By contrast, in vertebrates the clustered protocadherins (Pcdhs) provide analogous cell-surface diversity, but in this case generated through stochastic alternative promoter choice. Biophysical measurements with domain-deleted proteins showed that Pcdhs also interact in cis, through a membrane-proximal dimer interface involving extracellular cadherin domain 6 (EC6) and potentially EC5. The specificity-determining cell-cell recognition interface of Pcdhs involves domains EC1–4, as shown experimentally through mutagenesis analysis and suggested by mutation correlation analysis.

The γA1EC1–4 crystal structure contained four molecules in the asymmetric unit: Two of which are arranged in an EC1–4-mediated antiparallel dimer, with all four EC domains involved in the dimer interaction (chains A and B); and two are arranged in an EC2–3-mediated antiparallel dimer, in which EC1 and EC4 are not involved in the dimer interaction (chains C and D). The EC2–3 portion of the dimer interaction is very similar between the two dimers in the structure (RMSD = 0.98 Å over 415 Cα’s) and closely resembles the partial interaction observed in the previously published γA1EC1–3 structure (Nicoludis et al., 2015). The main difference between the two dimers in the γA1 crystal is therefore simply the presence or absence of the EC1:EC4 interaction. Since there are no protein domains filling the gap between EC1 and EC4 of chains C and D in the crystal, it is unclear why these domains do not interact. The fully engaged EC1–4-mediated dimer is similar to that of γB2EC1–5 and γB7EC1–4 and the published α- and β-Pcdh EC1–4-mediated dimers, involving the same interacting face of the molecule, however the RMSDs are quite large (4.3–5.0 Å; Figure 1—source data 3), highlighting the architectural differences between the γA1EC1–4 dimer and those of other Pcdh subtypes (Figure 1—source data 2–7). However, AUC of these fragments showed that all three were monomeric in solution, like the EC1–3 fragments of β1 and γC5. Given these data we conclude that the EC1:EC4 interaction is required for dimerization. The absence of this interaction in some of the γA crystal structures is therefore likely an artifact of crystallization, perhaps due to crystallization condition, although it does imply that the EC1:EC4 interaction is not particularly stable. While γB7 K338 forms a salt bridge with residue E41 in the γB7 homodimer, it would likely clash with γA1 R41 in a putative γA1:γB7 heterophilic complex.

>GNIRYSVPEETDKGSFVGSIAKDLGLETRELMERGIRIVSRGRSQLFSLNPRSGSLVTAGRIDREELCAQSTPCVVSFNILMEDEMKLLPIEVEIIDINDNTPQFQLEELELKMSEITTPGTRIPLPLGQDLDVGINSLQSYQLSANPHFSLDVQQGPEGPQQPEMVLQRPLDREKDAVHYLVLTASDGGSPIHSGTLQIHVQVVDVNDNPPAFTKAEYHVSVPENVPLGTRLLKVNATDPDEGANGRVTYSFHKVDHSVVRKFQLDAYTGELSNKEPLDFEEYKVYPMEIQAQDGAGLMARAKVLVTVLDVNDNAPEVGITSVTNTVPENFPPGTTIALISVHDQDADNNGHITCSIPGNLPFKLEKLVDNYYRLVTERTLDREQSSRHNITITATDQGTPPLSTQAHISLLVTDINDHHHHHHHH[4x]(3R)-3-HYDROXY-5,5-DIMETHYLHEXANOIC 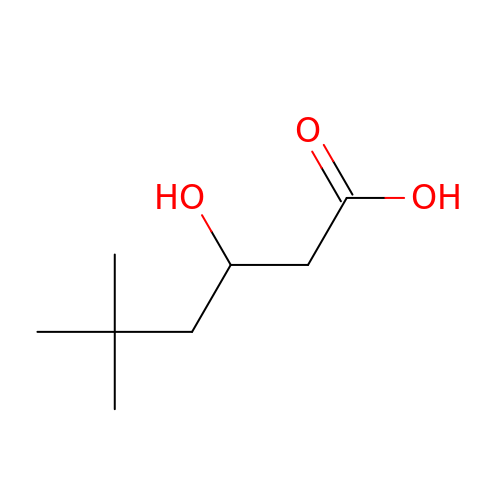ACID | C8 H16 O3 | PHACRADGRHURFF-LURJTMIESA-N>[6x]MSPLKNLVLDIDYNDAVVVIH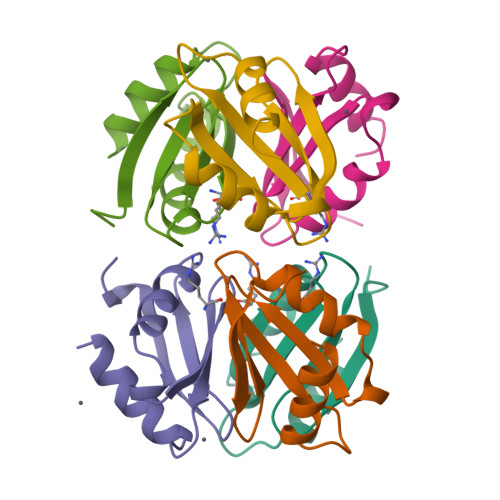TSPGAAQLIARLLDSLGKAEGILGTIAGDDTIFTTPANGFTVKDLYEAILELFDQEL Previously, the biosynthetic pathway of the immunosuppressive agent caerulomycin A (CRM A) from the marine actinomycete Actinoalloteichus cyanogriseus WH1-2216-6 has been identified, and the critical role of the (S)-selective ω-transaminase CrmG in the biosynthesis of CRM A has been reported. CrmG catalyzes amino acceptor caerulomycin M (CRM M) transformation to caerulomycin N (CRM N). Moreover, the activity of CrmG is insensitive to inhibition from ketone α-ketoglutarate or pyruvate.

The crystal structures of the apo form CrmG were determined to resolution 2.10 and 2.85 Å in space group I222 and C2, with one and two dimers in the asymmetric unit, respectively. Interestingly, in the structure of apo CrmG in I222 space group, the two catalytic pockets of CrmG dimer show completely different conformations. One catalytic pocket adopts the conformation similar with that of apo CrmG in C2 space group, in which the catalytic base K344 is exposed to solvent, here we name it “open” pocket; whereas the other catalytic pocket exhibits closed conformation, in which the G213-S232 loop acts like a lid covering on top of the catalytic K344, therefore K344 becomes inaccessible to the solvent. The closed pocket is more ordered than the open pocket. Residue W223 from the closed pocket forms a cation–π interaction with R451 from a symmetry-related molecule, indicating that the closed pocket might be stabilized by crystal packing. In addition, in the catalytic pocket of the closed apo form, residues S206-V212 form a helix, whereas this segment is a loop in both open apo form and cofactor-bound active form. However, in both open and closed apo pockets, the V317-I321 region adopts a more relaxed conformation, and Q318 occupies the position of the aromatic ring of PLP. To our knowledge, although numerous structures of ω-transaminase have been determined, here, we firstly report a closed form catalytic pocket of apo ω-transaminase with the active base inaccessible to the solvent. In apo CrmG, the active site is dynamic, which might switch between open and closed forms.

>[2x]MTHPSGEPVYADAVLNGWLTSMGLGVEYVRAEGNTVYYLDDEGREVPVLDHACGFGSLIFGHNHPEIIAHAKAALDAGTVVHAQLSRQPRANQISRILNDIMRRETGRDDRYNAIFANSGAEANEICMKHAELERQERITALFAEIDAELDTAREALTTGTATLDTASLPLVGGGAGDVDGVIADIHRHNDERRAERPLFLTLDGSFHGKLVGSIQLTQNEPWRTPFTALSSPARFLPADEPELIGKIVEDERRSVLTLSLDKDTVRVVERDFPVVAAIFVEPVRGGSGMKTVTPELAEELHRLRDTLGCPLVVDEVQTGIGRTGAFFGSALLGIRGDYYTLAKAIGGGIVKNSVALIRQDRFLPAMEVIHSSTFAKDGLSASIALKVLEMVEADGGRVYQRVRERGQRLEAMLESVRADHSDVVSAVWGTGLMLALELRDQSNATSQAIREKAAHGFLGYVLAGFLLREHHIRVLPAGPRSGFLRFSPSLYITDEEIDRTETALRSLFTALRDQDGDRLVLS> AHMNAGWVIGVDPDTSGALALLKPNQPPQVFDSPHLKVLVGKGVRKRLDAKAIVQLLKSFEAPIGTTVYVEQSTPYPQDGKQGWWSGGFGYGMWIGILVASGFSVIPVPSSAWKSEFQLTKERSNKDYSRQVASQLFPSLS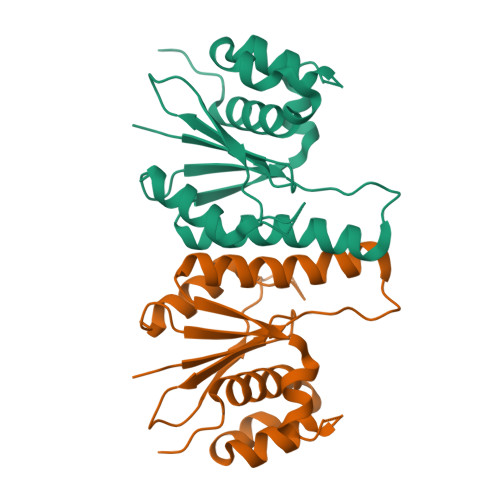SLLKRKKDHGRAEALLIAAYGKGIKINSDS6-azanyl-2-[[(2~{R},3~{S},4~{R},5~{R})-5-methoxy-3,4-bis(oxidanyl)oxolan-2-yl]methylamino]-3,7-dihydroimidazo[4,5-g]quinazolin-8-one 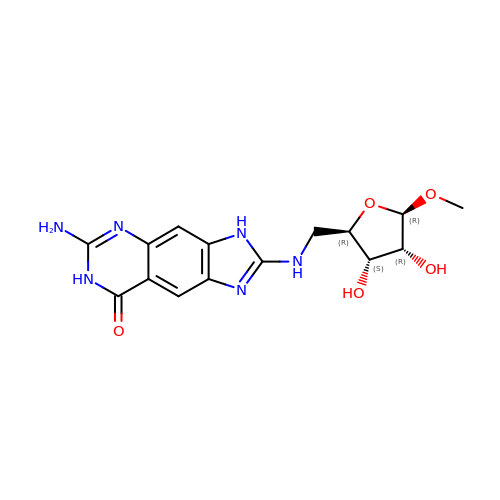| C15 H18 N6 O5 | ORQGUYZIZOFXKV-PRULPYPASA-N1-DECYL-3-TRIFLUORO ETHYL-SN-GLYCERO-2-PHOSPHOMETHANOL 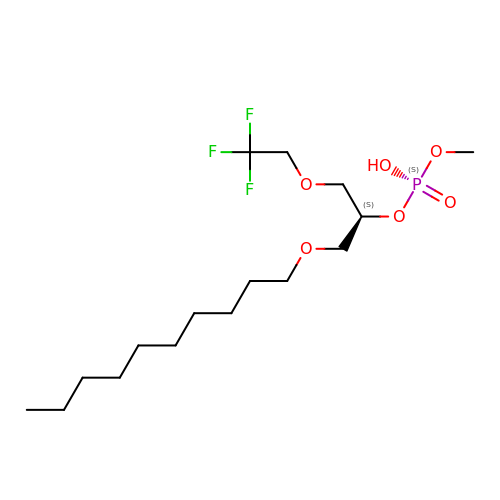| C16 H32 F3 O6 P | YBCDZAGHRGXDRX-HNNXBMFYSA-N> GPGTSTLSPGGGVTVFFHAIISLHFPFNPDLHKVFIRGGEEFGESKWDSNICELHYTRDLGHDRVLVEGIVCISKKHLDKYIPYKYVIYNGESFEYEFIYKHQQKKGEYVNRCLFIKSSLLGSGDWHQYYDIVYMKPHGRLQKVMNHITDGPRKDLVKGKQIAAALMLDSTFSILQTWDTINLNSFFTQFEQFCFVLQQPMIYEGQAQLWTDLQYREKEVKRYLWQHLKKHVVPLPDGKSTDFLPVDCPVRSKLKTGLIVLFVVEKIELLLEGSLDWLCHLLTSDASSPDEFHRDLSHILGIPQSWRLYLVNLCQRCMDTRTYTWLGALPVLHCCMELAPRHKDAWRQPEDTWAALEGLSFSPFREQMLDTSSLLQFMREKQHLLSIDEPLFRSWFSLLPLSHLVMYMENFIEHLGRFPAHILDCLSGIYYRLPGLEQVLNTQDVQDVQNVQNILEMLLRLLDTYRDKIPEEALSPSYLTVCLKLHEAICSSTKLLKFYELPALSAEIVCRMIRLLSLVDSAGQRDETGNNSVQTVFQGTLAATKRWLREVFTKNMLTSSGASFTYVKEIEVWRRLVEIQFPAEHGWKESLLGDMEWRLTKEEPLSQITAYCNSCWDTKGLEDSVAKTFEKCIIEAVSSACQSQTSILQGFSYSDLRKFGIVLSAVITKSWPRTADNFDDILKHLLTLADVKHVFRLCGTDEKILANVTEDAKRLIAVADSVLTKVVGDLLSGTILVGQLELIIKHKNQFLDIWQLREKSLSPQDEQCAVEEALDWRREELLLLKKEKRCVDSLLKMCGNVKHLIQVDFGVLAVRHSQDLSSKRLNDTVTVRLSTSSNSQRATHYHLSSQVQEMAGKIDLLRDSHIFQLFWREAAEPLSEPKEDQEAAELLSEPEEESERHILELEEVYDYLYQPSYRKFIKLHQDLKSGEVTLAEIDVIFKDFVNKYTDLDSELKIMCTVDHQDQRDWIKDRVEQIKEYHHLHQAVHAAKVILQVKESLGLNGDFSVLNTLLNFTDNFDDFRRETLDQINQELIQAKKLLQDISEARCKGLQALSLRKEFICWVREALGGINELKVFVDLASISAGENDIDVDRVACFHDAVQGYASLLFKLDPSVDFSAFMKHLKKLWKALDKDQYLPRKLCDSARNLEWLKTVNESHGSVERSSLTLATAINQRGIYVIQAPKGGQKISPDTVLHLILPESPGSHEESREYSLEEVKELLNKLMLMSGKKDRNNTEVERFSEVFCSVQRLSQAFIDLHSAGNMLFRTWIAMAYCSPKQGVSLQMDFGLDLVTELKEGGDVTELLAALCRQMEHFLDSWKRFVTQKRMEHFYLNFYTAEQLVYLSTELRKQPPSDAALTMLSFIKSNCTLRDVLRASVGCGSEAARYRMRRVMEELPLMLLSEFSLVDKLRIIMEQSMRCLPAFLPDCLDLETLGHCLAHLAGMGGSPVERCLPRGLQVGQPNLVVCGHSEVLPAALAVYMQTPSQPLPTYDEVLLCTPATTFEEVALLLRRCLTLGSLGHKVYSLLFADQLSYEVARQAEELFHNLCTQQHREDYQLVMVCDGDWEHCYLPSAFSQHKVFVTPQAPLEAIQAYLAGHYRVPKQTLSAAAVFNDRLCVGIVASERAGVGKSLYVKRLHDKMKMQLNVKNVPLKTIRLIDPQVDESRVLGALLPFLDAQYQKVPVLFHLDVTSSVQTGIWVFLFKLLILQYLMDINGKMWLRNPCHLYIVEILERRTSVPSRSSSALRTRVPQFSFLDIFPKVTCRPPKEVIDMELSALRSDTEPGMDLWEFCSETFQRPYQYLRRFNQNQDLDTFQYQEGSVEGTPEECLQHFLFHCGVINPSWSELRNFARFLNYQLRDCEASLFCNPSFIGDTLRGFKKFVVTFMIFMARDFATPSLHTSDQSPGKHMVTMDGVREEDLAPFSLRKRWESEPHPYVFFNDDHTTMTFIGFHLQPNINGSVDAISHLTGKVIKRDVMTRDLYQGLLLQRVPFNVDFDKLPRHKKLERLCLTLGIPQATDPDKTYELTTDNMLKILAIEMRFRCGIPVIIMGETGCGKTRLIKFLSDLRRGGTNADTIKLVKVHGGTTADMIYSRVREAENVAFANKDQHQLDTILFFDEANTTEAISCIKEVLCDHMVDGQPLAEDSGLHIIAACNPYRKHSEEMICRLESAGLGYRVSMEETADRLGSIPLRQLVYRVHALPPSLIPLVWDFGQLSDVAEKLYIQQIVQRLVESISLDENGTRVITEVLCASQGFMRKTEDECSFVSLRDVERCVKVFRWFHEHSAMLLAQLNAFLSKSSVSKNHTERDPVLWSLMLAIGVCYHASLEKKDSYRKAIARFFPKPYDDSRLLLDEITRAQDLFLDGVPLRKTIAKNLALKENVFMMVVCIELKIPLFLVGKPGSSKSLAKTIVADAMQGPAAYSDLFRSLKQVHLVSFQCSPHSTPQGIISTFRQCARFQQGKDLQQYVSVVVLDEVGLAEDSPKMPLKTLHPLLEDGCIEDDPAPHKKVGFVGISNWALDPAKMNRGIFVSRGSPNETELIESAKGICSSDILVQDRVQGYFASFAKAYETVCKRQDKEFFGLRDYYSLIKMVFAAAKASNRKPSPQDIAQAVLRNFSGKDDIQALDIFLANLPEAKCSEEVSPMQLIKQNIFGPSQKVPGGEQEDAESRYLLVLTKNYVALQILQQTFFEGDQQPEIIFGSGFPKDQEYTQLCRNINRVKICMETGKMVLLLNLQNLYESLYDALNQYYVHLGGQKYVDLGLGTHRVKCRVHPNFRLIVIEEKDVVYKHFPIPLINRLEKHYLDINTVLEKWQKSIVEELCAWVEKFINVKAHHFQKRHKYSPSDVFIGYHSDACASVVLQVIERQGPRALTEELHQKVSEEAKSILLNCATPDAVVRLSAYSLGGFAAEWLSQEYFHRQRHNSFADFLQAHLHTADLERHAIFTEITTFSRLLTSHDCEILESEVTGRAPKPTLLWLQQFDTEYSFLKEVRNCLTN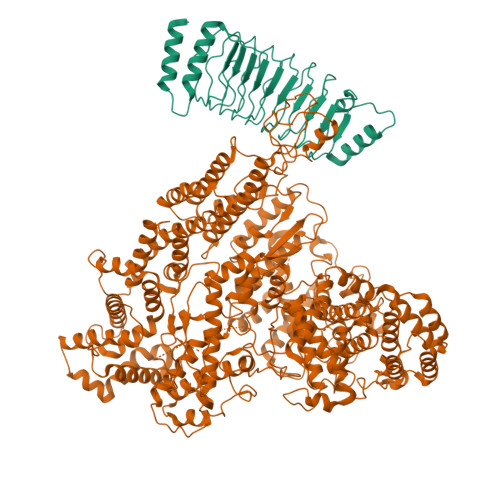TAKCKILIFQTDFEDGIRSAQLIASAKYSVINEINKIRENEDRIFVYFITKLSRVGRGTAYVGFHGGLWQSVHIDDLRRSTLMVSDVTRLQHVTISQLFAPGDLPELGLEHRAEDGHEEAMETEASTSGEVAEVAEEAMETESSEKVGKETSELGGSDVSILDTTRLLRSCVQSAVGMLRDQNESCTRNMRRVVLLLGLLNEDDACHASFLRVSKMRLSVFLKKQEESQFHPLEWLAREACNQDALQEAGTFRHTLWKRVQGAVTPLLASMISFIDRDGNLELLTRPDTPPWARDLWMFIFSDTMLLNIPLVMNNERHKGEMAYIVVQNHMNLSENASNNVPFSWKIKDYLEELWVQAQYITDAEGLPKKFVDIFQQTPLGRFLAQLHGEPQQELLQCYLKDFILLTMRVSTEEELKFLQMALWSCTRKLKAASEAPEEEVSLPWVHLAYQRFRSRLQNFSRILTIYPQVLHSLMEARWNHELAGCEMTLDAFAAMACTEMLTRNTLKPSPQAWLQLVKNLSMPLELICSDEHMQGSGSLAQAVIREVRAQWSRIFSTALFVEHVLLGTESRVPELQGLVTEHVFLLDKCLRENSDVKTHGPFEAVMRTLCECKETASKTLSRFGIQPCSICLGDAKDPVCLPCDHVHCLRCLRAWFASEQMICPYCLTALPDEFSPAVSQAHREAIEKHARFRQMCNSFFVDLVSTICFKDNAPPEKEVIESLLSLLFVQKGRLRDAAQRHCEHTKSLSPFNDVVDKTPVIRSVILKLLLKYSFHDVKDYIQEYLTLLKKKAFITEDKTELYMLFINCLEDSILEKTSAYSRNDELNHLEEEGRFLKAYSPASRGREPANEASVEYLQEVARIRLCLDRAADFLSEPEGGPEMAKEKQCYLQQVKQFCIRVENDWHRVYLVRKLSSQRGMEFVQGLSKPGRPHQWVFPKDVVKQQGLRQDHPGQMDRYLVYGDEYKALRDAVAKAVLECKPLGIKTALKACKTPQSQQSAYFLLTLFREVAILYRSHNASLHPTPEQCEAVSKFIGECKILSPPDISRFATSLVDNSVPLLRAGPSDSNLDGTVTEMAIHAAAVLLCGQNELLEPLKNLAFSPATMAHAFLPTMPEDLLAQARRWKGLERVHWYTCPNGHPCSVGECGRPMEQSICIDCHAPIGGIDHKPRDGFHLVKDKADRTQTGHVLGNPQRRDVVTCDRGLPPVVFLLIRLLTHLALLLGASQSSQALINIIKPPVRDPKGFLQQHILKDLEQLAKMLGHSADETIGVVHLVLRRLLQEQHQLSSRRLLNFDTELSTKEMRNNWEKEIAAVISPELEHLDKTLPTMNNLISQDKRISSNPVAKIIYGDPVTFLPHLPRKSVVHCSKIWSCRKRITVEYLQHIVEQKNGKERVPILWHFLQKEAELRLVKFLPEILALQRDLVKQFQNVQQVEYSSIRGFLSKHSSDGLRQLLHNRITVFLSTWNKLRRSLETNGEINLPKDYCSTDLDLDTEFEILLPRRRGLGLCATALVSYLIRLHNEIVYAVEKLSKENNSYSVDAAEVTELHVISYEVERDLTPLILSNCQYQVEEGRETVQEFDLEKIQRQIVSRFLQGKPRLSLKGIPTLVYRHDWNYEHLFMDIKNKMAQDSLPSSVISAISGQLQSYSDACEVLSVVEVTLGFLSTAGGDPNMQLNVYTQDILQMGDQTIHVLKALNRCQLKHTIALWQFLSAHKSEQLLRLHKEPFGEISSRYKADLSPENAKLLSTFLNQTGLDAFLLELHEMIILKLKNPQTQTEERFRPQWSLRDTLVSYMQTKESEILPEMASQFPEEILLASCVSVWKTAAVLKWNREMR;> GPGSMIKSTNIQAIGSGIMHQINNVYSLTPLSLPMELTPSMNEFYLKTWSEWEKNGTPGEQRNIAFNRLKICLQNQEAELNLSELDLKTLPDLPPQITTLEIRKNLLTHLPDLPPMLKVIHAQFNQLESLPALPETLEELNAGDNKIKELPFLPENLTHLRVHNNRLHILPLLPPELKLLVVSGNRLDSIPPFPDKLEGLALANNFIEQLPELPFSMNRAVLMNNNLTTLPESVLRLAQNAFVNVAGNPLSGHTMRTLQQITTGPDYSGPRIFFSMGNSATISAPEHSLADAVTAWFPENKQSDVSQIWHAFEHEEHANTFSAFLDRLSDTVSARNTSGFREQVAAWLEKLSASAELRQQSFAVAADATESCEDRVALTWNNLRKTLLVHQASEGLFDNDTGALLSLGREMFRLEILEDIARDKVRTLHFVDEIEVYLAFQTMLAEKLQLSTAVKEMRFYGVSGVTANDLRTAEAMVRSREENEFTDWFSLWGPWHAVLKRTEADRWAQAEEQKYEMLENEYSQRVADRLKASGLSGDADAEREAGAQVMRETEQQIYRQLTDEVLALRLSENGSNHIA> MGSRAICIQRVAPPCFEASQVKKIKTVGSFLVNTRSKRRRSTGVKCSSIADYIGGDLVKPDIGQWLQDVEEHKAIAIYAPHEGGYEGRYLNRLKMQGYYFLDISARGLGDPETTLLKNYPVCPAHLGKQPIARWYYPPEVDYRLAALPPSAKGLVVWVLEAKVLSKSELQFLAL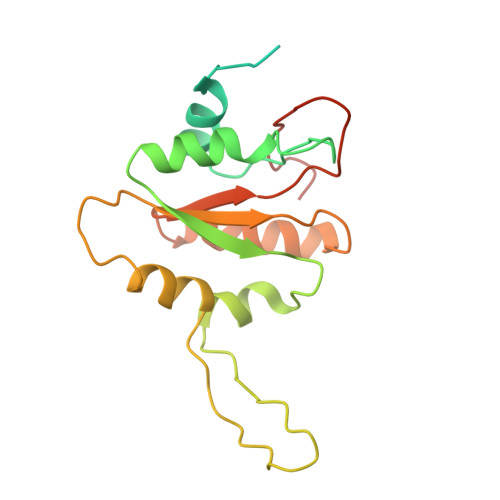LPSLRPNVRVIAECGNWRKFVWKPLAEIANLAAQE The PH domain-containing protein Slm1 from budding yeast Saccharomyces cerevisiae is required for actin cytoskeleton polarization and cell growth. The PH domain-containing protein Slm1 from S. cerevisiae is a component of the target of rapamycin complex 2 (TORC2) signaling pathway. We have previously reported that in vitro, the Slm1-PH domain (Slm1-PH) interacts with liposomes containing PtdIns(4,5)P2 and DHS-1P cooperatively. The core of each monomer consists of seven antiparallel β-strands with a C-terminal amphipathic α-helix connected via a long and flexible loop.

The results presented here include: (i) the apo structure of Slm1-PH that we resolved at 1.76 Å resolution; (ii) one structure with phosphoserine at 1.68 Å resolution; and (iii) two structures of Slm1-PH in complex with Ins(4)P at 1.4 and 1.8 Å resolution. We previously reported a structure for the apo Slm1-PH (at 2.0 Å) that depicted only part of the non-canonical binding site. As the interactions between the two molecules involve the backbone of β1-β2 and no specific side-chain residue, this probably represents a crystallographic packing artifact. Compared with our previously published structure at 2 Å, our new apo structure clearly visualizes the full β5-β6 loop, which plays a key role in accommodating ligand molecules in the non-canonical binding site (see below). Interestingly for all four structures, much of the binding space in the canonical binding site is occupied by the β5-β6 loop of the neighboring molecule. The long β5-β6 loop occupied part of the space at the canonical binding cavity, making it less available for ligand binding.

>PFTEIKSGFLERRSKFLKSYSKGYYVLTPNFLHEFKTADRKKDLVPVMSLALSECTVTEHSRKNSTSSPNSTGSDAKFVLHAKQNGIIRRGHNWVFKADSYESMMSWFDNLKILTSTS[4x]>[2x]TELTKCKVSHAIKDIDGYQGISLLEWACV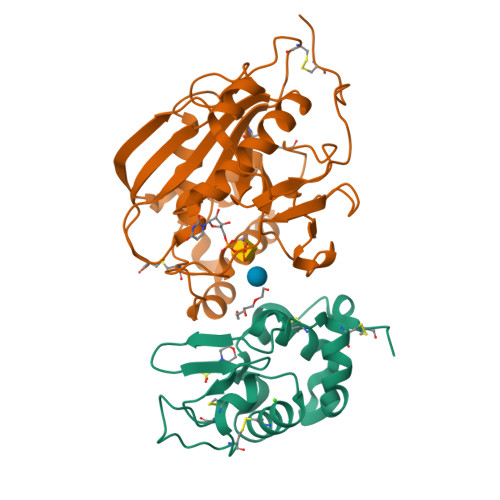LFHTSGYDTQAVVNDNGSTEYGLFQISDRFWCKSSEFPESENICGISCDKLLDDELDDDIACAKKILAIKGIDYWKAYKPMCSEKLEQWRCEKP;>[2x]ASMTGGQQMGRGSSLTACPEESPLLVGPMLIEFNIPVDLKLVEQQNPKVKLGGRYTPMDCISPHKVAIIIPFRNRQEHLKYWLYYLHPILQRQQLDYGIYVINQAGESMFNRAKLLNVGFKEALKDYDYNCFVFSDVDLIPMNDHNTYRCFSQPRHISVAMDKFGFSLPYVQYFGGVSALSKQQFLSINGFPNNYCGWGGEDDDIYNRLAFRGMSVSRPNAVIGKTRMIRHSRDKKNEPNPQRFDRIAHTKETMLSDGLNSLTYMVLEVQRYPLYTKITVDIGTCS> MREEPSSAQLFKPLKVGRCHLQHRMIMAPTTRFRADGQGVPLPFVQEYYGQRASVPGTLLITEATDITPKAMGYKHVPGIWSEPQREAWREIVSRVHSKKCFIFCQLWATGRAADPDVLADMKDLISSSAVPVEEKGPLPRALTEDEIQQCIADFAQAARNAINAGFDGVEIHGANGYLIDQFTQKSCNHRQDRWGGSIENRARFAVEVTRAVIEAVGADRVGVKLSPYSQYLGMGTMDELVPQFEYLIAQMRRLDVAYLHLANSRWLDEEKPHPDPNHEVFVRVWGQS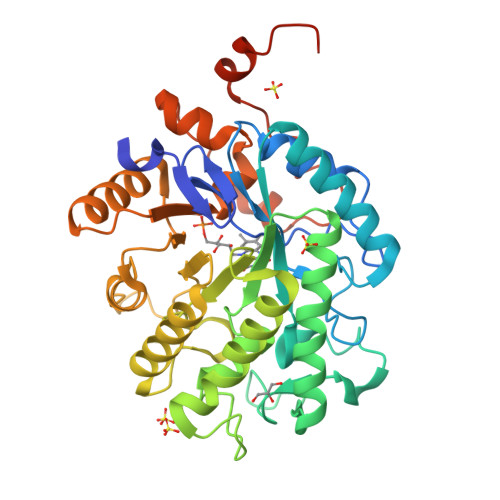SPILLAGGYDAASAEKVTEQMAAATYTNVAIAFGRYFISTPDLPFRVMAGIQLQKYDRASFYSTLSREGYLDYPFSAEYMALHNFPVASGKLAAALEHHHHHH>MVKTQRVVITPGEPAGIGPDLVVQLAQREWPVELVVCADATLLTNRAAMLGLPLTLRPYSPNSPAQPQT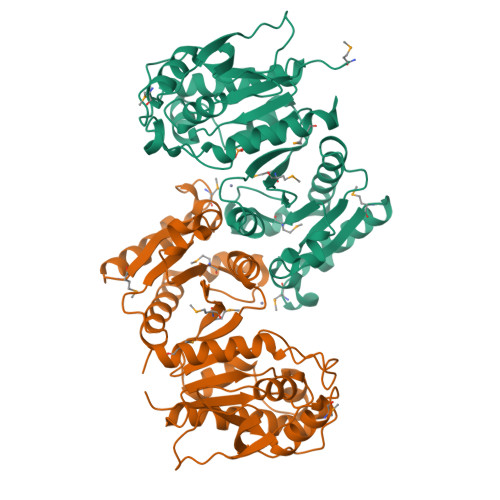AGTLTLLPVALRAPVTAGQLAVENGHYVVETLARACDGCLNGEFAALITGPVHKGVINDAGIPFTGHTEFFEERSQAKKVVMMLATEELRVALATTHLPLRDIADAITPALLHEVIAILHHDLRTKFGIAEPRILVCGLNPHAGEGGHMGTEEIDTIIPVLNELRAQGMKLNGPLPADTLFQPKYLDNADAVLAMYHDQGLPVLKYQGFGRGVNITLGLPFIRTSVDHGTALELAGRGKADVGSFITALNLAIKMIVNTQ[2x]> MAHHHHHHMNKPVTPKTPKLRSRAWFDNPDDVDMTALYLERYMNYGLSQEELQSGRPIIGIAQTGSDLSPCNRHHLEL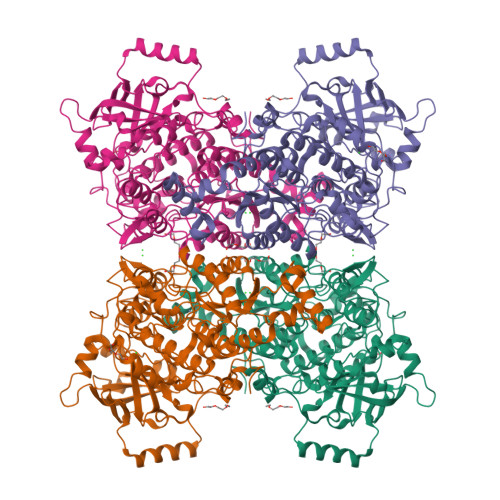AKRVRDGVREAGGIVIEFPVHPIQETGKRPTAGLDRNLAYLGLVEVLYGYPLDGVVLTIGCDKTTPACLMAAATVNIPAIALSVGPMLNGWFRGERTGSGTIVWKARELLAKGEIDYQGFVKLVASSAPSTGYCNTMGTATTMNSLAEALGMQLPGSAAIPAPYRDRQEVAYLMGRRIVEMVHEDLKPSDILTKEAFINAIRVNSAIGGSTNAPIHLNALARHIGVELTVDDWQKYGEEIPLLVNLQPAGEYLGEDYYHAGGVPAVVNQLMGQGLIHEDAITVNGKTIGENCKNATIEDGNVIKTYDQPLKKHAGFRVLRGNLFSSAIMKLSVISDEFRNRYLSDAKDPNAFEGKAVVFDGPEDYHHRIDDPALEIDEHTVLFMRGAGPIGYPGAAEVVNMRAPDYLLKKGITSLPCIGDGRQSGTSGSPSILNASPEAAAGGGLAILKTGDRVRIDLGRGTADILISDEELAERRKALEAVGGYKYPESQTPWQEIQRAVIGQMETGAVLENAVKYQDIAHTRGLPRDNH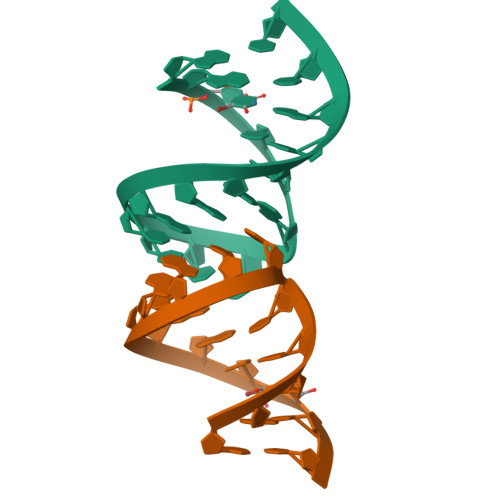> GGUCGGUCCCAGACGACC;> GGAGCCUGGGAGCUCC> SFNLAPLGRRR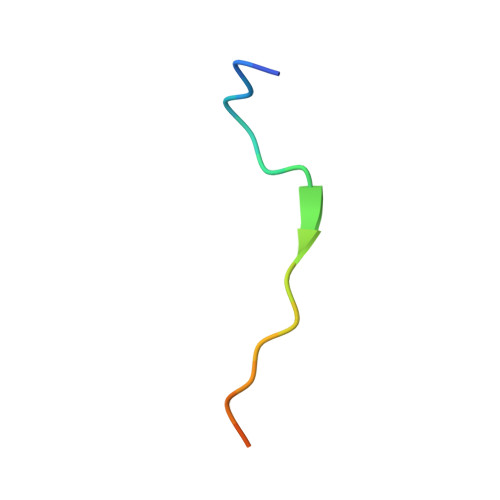VQSQWAST>[2x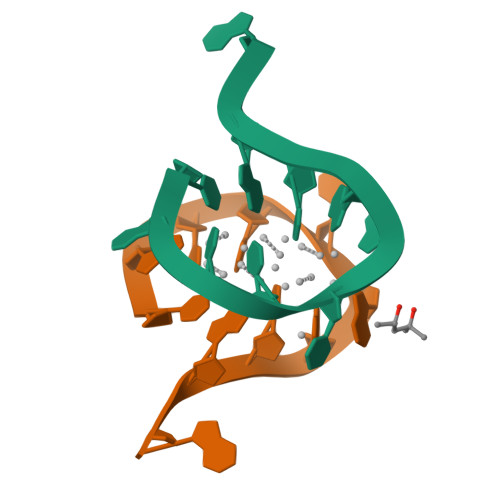]CACCTAICGA> MDNLLRHLKISKEQITPVVLVVGDPGRVDKIKVVCDSYVDLAYNREYKSVECHYKGQKFLCVSHGVGSAGCAVCFEELCQNGAKVIIRAGSCGSLQPDLIKRGDICICNAAVREDRVSHLLIHGDFPAVGDFDVYDTLNKCA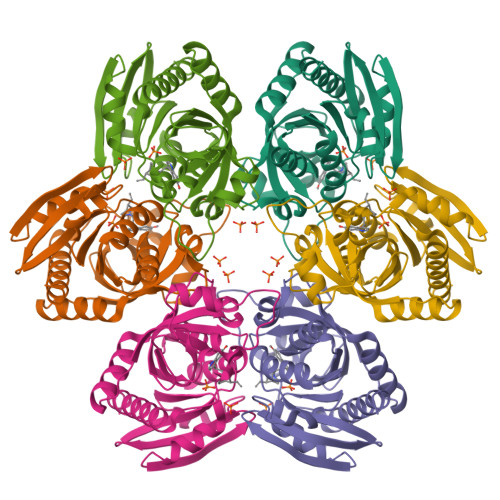QELNVPVFNGISVSSDMYYPNKIIPSRLEDYSKANAAVVEMELATLMVIGTLRKVKTGGILIVDGCPFKWDEGDFDNNLVPHQLENMIKIALGACAKLATKYA>[4x]KSFVITDPRLPDNPIIFA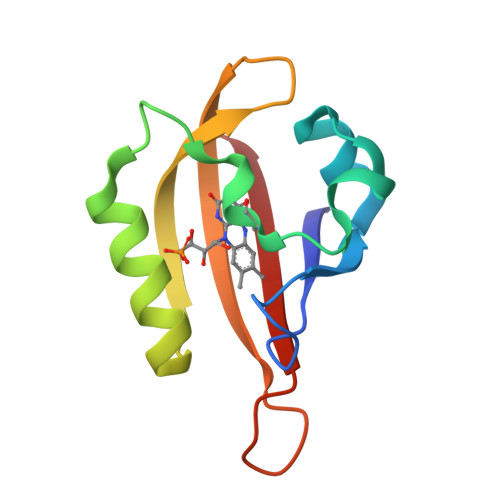SDRFLELTEYTREEVLGNNCRFLQGRGTDRKAVQLIRDAVKEQRDVTVQVLNYTKGGRAFWNLFHLQVMRDENGDVQYFIGVQQEM In this work, we describe the identification and characterization of a Trypanosoma brucei FH receptor (FHR). FH blocks the complement cascade by accelerating the decay of C3 convertase (C3bBb), thus reducing C3b production, and by acting as a co-factor for factor I, which cleaves and inactivates C3b4. FH is composed of 20 tandem complement control protein (CCP) domains with 6, 7 and 20 binding self-cell-negative surface markers, whereas 1–4 and 19 bind C3b5–8. Here we have identified and characterized FHR, a receptor that binds FH in a manner that would enable FH to negatively regulate C3b and C3bBb preventing MAC formation.

The structure of the FHR bound to FH domain 5 was determined by X-ray crystallography. The ordered part of the FHR structure observed in the crystal starts at the mature N terminus (residue 25) and ends 14 residues before the predicted mature C terminus and GPI anchor (residue 237). FHR is an elongated three-helical bundle of ~90 Å similar to other trypanosome receptors, but has evolved a binding pocket for FH domain 5 through spreading apart of the membrane-distal ends of the long second and third helices. Domain 5 has a CCP fold as expected, with its N terminus pointing away from the plasma membrane. Two copies of FHR and two of FH domain 5 were present in the asymmetric unit of the crystal with each receptor contacting both copies of domain 5. Mutant 2 FHR resolved which interaction was representative of the physiological complex and which was due to crystal packing. That is, mutant 2 contained mutations E31A and Q34A within one of the possible interfaces; these alterations disrupted the receptor-ligand interaction by pulldown and also by SPR analysis, thus confirming that the interaction is mediated by the binding site containing these residues shown in Fig. 3. The single predicted N-linked glycosylation site in FHR is located at the extreme membrane-distal tip of the molecule and in this position the oligosaccharide could potentially reduce antibody accessibility of FHR molecules embedded in the trypanosome surface coat without interfering with FH binding. The location of the FH-binding site is informative about the mode of action; by binding FH domain 5 at a site distal to the plasma membrane, FH domains 1–4 are located in the likely location of deposited C3b at the periphery on the cell surface coat. The highest affinity interaction, with a similar KD to full-length FH, was between FHR and FH domains 4-5-6 with a KD of 167 nM and the KD for binding to domain 5 alone was 562 nM.

>[2x]GPNDNLEAELEQTKALCEVAKQLRKLPLLTEERRFEAVGALEESKKAAKEGKKAAKRAEAGAVGGTSEQQQAAKRAREAATVAYEASVRAEAAAMEVKRFARALDSFESEYESVFSGLLRGAAEHGGNETIKQLAKECATAVADDVTPEALTRAAHNLRGLYMQDFAEEYLQEANEAANKLEELQKATAETVRAADAADDAKSEAQEEAAQFPEIDDDDSDEDKEDEAS;>GEITCDPPRIPNGVYRPELSKYRGQDKITYECKKGFFPEIRGTDATCTRDGWVPVPRCAWK[2x]1-[(10~{b}~{S})-6-oxidanylidene-2,3,4,10~{b}-tetrahydro-1~{H}-pyrido[2,1-a]isoindol-10-yl]-3-[4-[1-[2-(1,2,3,4-tetrahydroacridin-9-ylamino)ethyl]-1,2,3-triazol-4-yl]pyridin-2-yl]urea 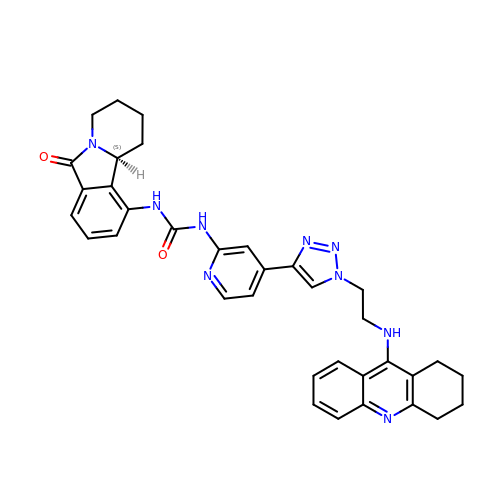| C35 H35 N9 O2 | BNBWNJAILLASJW-PMERELPUSA-N> SAWRKAGISYAAYLNVAAQAIRSSLKTELQTASVLNRSQTDAF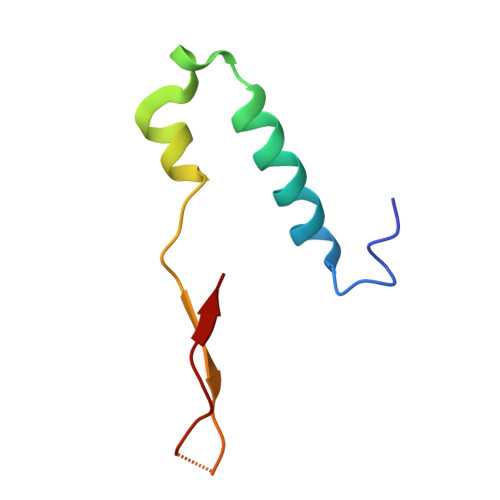YTQYKNGTAASEPTPITK> 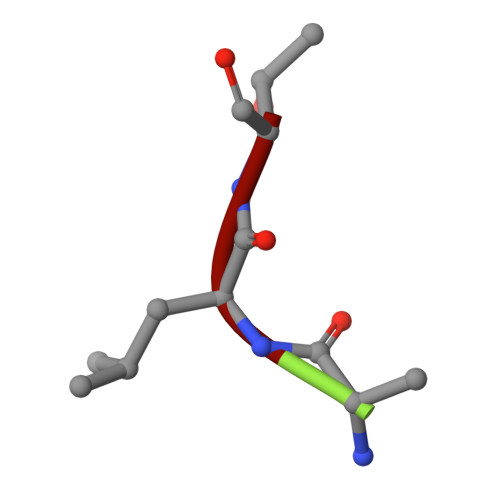ALT>[3x]MHHHHHHSSGLVPRGSMILHAQAKHGKPGLPWLVFLHGFSGDCHEWQEVGEAFADYSRLYVDLPGHGGSAAISVDGFDDVTDLLRKTLVSYNILDFWLVGFSLGGRVAMMAACQGLAGLCGVIVEGGHPGLQNAEQRAERQRSDRQWVQRFLTEPL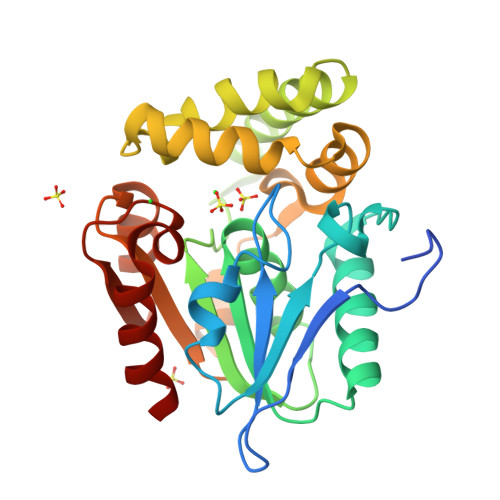TAVFADWYQQPVFASLNDDQRRELVALRSNNNGATLAAMLEATSLAVQPDLRANLSARTFAFYYLCGERDSKFRALAAELAADCHVIPRAGHNAHRENPAGVIASLAQILRF>ETGDKPLGETGTTGFQICKNALKLPVLEVLPGGGWDNLRNVDMGRVMDLTYTNCKTTEDGQYIIPDEVYTIPQKESNLEMNSEVLESWMNYQSTTSLSINTELALFSRVNGKFSTEFQRMKTLQVKDQAVTTRVQVRNRIYTVKTTPTSELSLGFTKALMDICDQLEKNQTKMATYLAELLILNYGTHVITSVDAGAALVQEDHVRSSFLLDNQNSQNTVTASAGIAFLNIVNFKVETDYISQTSLTKDYLSNRTNSRVQSFGGVPFYPGITLETWQK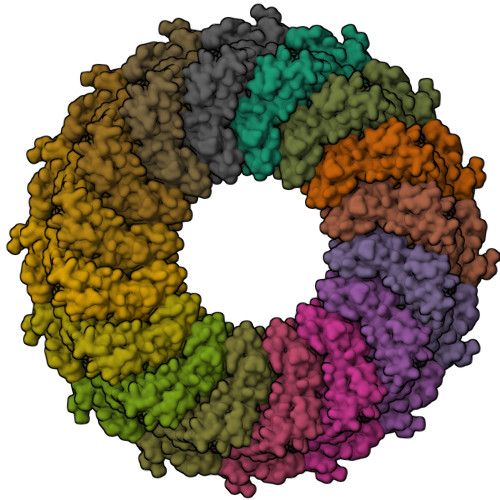GITNHLVAIDRAGLPLHFFIKPDKLPGLPGPLVKKLSKTVETAVRHYYTFNTHPGCTNVDSPNFNFQANMDDDSCDAKVTNFTFGGVYQECTELSGDVLCQNLEQKNLLTGDFSCPPGYSPVHLLSQTHEEGYSRLECKKKCTLKIFCKTVCEDVFRVAKAEFRAYWCVAAGQVPDNSGLLFGGVFTDKTINPMTNAQSCPAGYIPLNLFESLKVCVSLDYELGFKFSVPFGGFFSCIMGNPLVNSDTAKDVRAPSLKKCPGGFSQHLAVISDGCQVSYCVKAGIFTGGSLLPVRLPPYTKPPLMSQVATNTVIVTNSETARSWIKDPQTNQWKLGEPLELRRAMTVIHGDSNGMSGGGTETSQVAPA[16x]> MVAKGRIIRVTGPLVVADGMKGAKMYEVVRVGELGLIGEIIRLEGDKAVIQVYEETAGVRPGEPVVGTGASLSVELGPGLLTSIYDGIQRPLEVIREKTGDFIARGVTAPALPRDKKWHFIPKAKVGDKVVGGDIIGEVPETSIIVHKIMVPPGIEGEIVEIAEEGDYTIEEVIAKVKTPSGEIKELKMYQRWPVRVKRPYKEKLPPEVPLITGQRVIDTFFPQAKGGTAAIPGPFASGKTVTQHQLAKWSDAQVVIYIGCGERGNEMTDVLEEFPKLKDPKTGKPLMERTVLIANTSNMPVAAREASIYTGITIAEYFRDMGYDVALMADSTSRWAEALREISGRLEEMPGEEGYPAYLASKLAEFYERAGRVVTLGSDYRVGSVSVIGAVSPPGGDFSEPVVQNTLRVVKVFWALDADLARRRHFPAINWLTSYSLYVDAVKDWWHKNIDPEWKAMRDKAMALLQKESELQEIVRIVGPDALPERERAILLVARML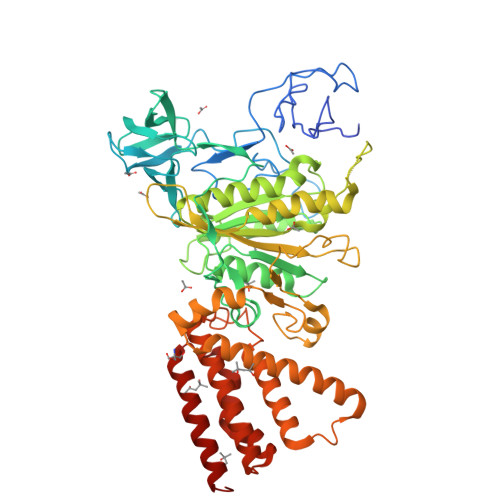REDYLQQDAFDEVDTYCPPEKQVTMMRVLLNFYDKTMEAINRGVPLEEIAKLPVREEIGRMKFERDVSKIRSLIDKTNEQFEELFKKYGA Supporting this hypothesis, we here determined the fibril structure of two AMPs from amphibians, uperin 3.5 and aurein 3.3, by cryogenic electron microscopy (cryo-EM), revealing amyloid cross-β fibrils of mated β-sheets at atomic resolution. For both of the studied ffAMPs, cryo-EM data unambiguously prove an amyloid cross-β structure comprised of β-sheets with tightly coupled dry interfaces and strands perpendicular to the fibril axis. Despite the dissimilarity in lateral fibril structure and the difference of extended versus kinked β-sheets, the 17-residue ffAMPs uperin 3.5 and aurein 3.3 are remarkably similar in their residue composition. Overall, compared to other amyloids, the sequence content of the two AMPs indicates a dominant apolar and positively charged nature, which fits the functional interactions with negatively charged bacterial membranes.

A recently developed computational screen aimed to identify fibril-forming AMPs (ffAMPs) additional to uperin 3.5 found fourteen new sequences, including aurein 3.3, another amphibian AMP secreted by Ranoidea raniformis (Southern bell frog). In contrast to the case of uperin 3.5, we did not observe any pronounced polymorphism of fibrils formed by the antimicrobial peptide aurein 3.3. Two of those (chains E, F) are arranged in a cross-like shape conforming to C21 screw-symmetry along the fibril axis and form kinked β-sheets in their inner section which closely meet at a roughly 90° bend near Gly11. Wrapped around this inner cross are four more strands of mutually similar conformation, each having a sharp in-plane kink near the outward-facing His12 residue, which is enabled by Gly11 leaving a void into which Val14 can fold. The outer chains, in particular C and D, cross the fibril normal at an unusually large angle and are strongly bent in the plane of their respective β-sheet, which, together with the screw symmetry of the inner cross, leads to a complex staggered structure of the fibril without well-defined rungs. The overall packing of the aurein 3.3 fibril is highly dense, with the SASA buried for a single layer (fibril cross-section of six lateral chains) covering 9802 Å2, which is 83% of the total area of this layer. In the outer chains C and D, the C-terminal part of the kinked β-sheet forms tightly mated β-sheet interactions with the C-terminal part of the inner chain F, overall showing a stable interface of three short β-sheets, resembling lateral association between β-sheets in the crystal structures of short amyloid segments. Overall, the lateral association of β-sheets in the aurein 3.3 fibril shows very few potential polar interactions and is mostly stabilized by van der Waals forces. Here we show the cryo-EM structure of aurein 3.3, revealing a cross-β fibril with kinked β-sheets. Such sharp kinks in the peptide backbone are the hallmark of Low-complexity Amyloid-like Reversible Kinked Segments (LARKS) within functional amyloids.

>GLFDIVKKIAGHIVSSI[18x]> SELIVNVINGPNLGRLGRREPAVYGGTTHDELVALIEREAAELGLKAVVRQSDSEA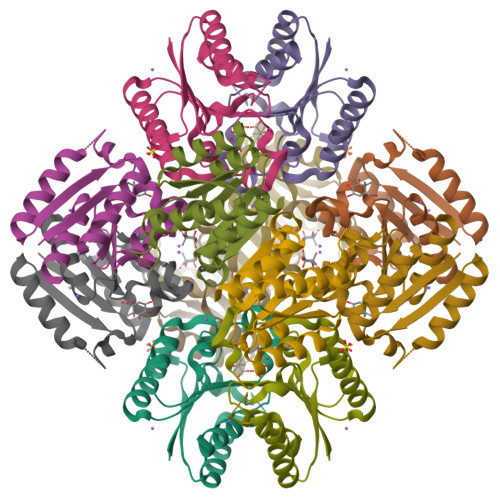QLLDWIHQAADAAEPVILNAGGLTHTSVALRDACAELSAPLIEVHISNVHAREEFRRHSYLSPIATGVIVGLGIQGYLLALRYLAEHVGT> MIKNILGLALGTNSIGWALVKQDFENKQGEILGMGSRIIPMSQDILGDFGKGNSVSQTAERTKYRSVRRLRERFLLRRERLHRVLYILNFLPEHYASQIDFEKRLGKFKVETEPKLVWKNTDGQFSFLFQNSFNEMLEDFKAAGQELKIPYDWTIYHLRKKAISQKIEKEELAWILLNFNHKRGYYQLRGEDFEEEKDKTFVRLKVDRIVDSGENVKGKILYDVYFENGWKYDKQVVKTEDWVDRTKEFIVSESILKNGETKRTFKAVDSEKDWIAIKTKTEQEIEHSHKTVGTYIYETLLQNPKQKIKGKLVRTIERKFYKEELRQILEKQKEFHQELQSDDLYNDCIRELYRNNEVHQLTLRKKDFVHLFMEDIIFYQRPLRSQKSSVSNCTLEFRKYKGENGAEHTQYLKAIPKSNPYYQEFRLWQWIFNLNLYTKDNDENVTKVFLNTTQDFENLFEFLNTRKEVDQKALLKHFKLNEKTHRWNFVEDKKYPCNETKTMISSRLDKVENISDDFLTRDIEQKIWHIIYSVNDKVEYEKALKSFARKHHLDESSFFEAFRKFPPFKSEYGSFSEKAIKKLLPLMRLGKYWNYAEIDKYSRERIQKIITGEYDENIKDKVREKSVHLTIENDFQGLQLWLAQYIVYGRHSEASMIGKWNSANDLEVFLKDFKQHSLRNPIVEQVITETLRVVKDIWLKYGNGTKDFFNEIHIELGREMKLPADDRKKLTNQITENENTNLRIKALLAEMMNDHSVENVRPFSPMQQEILKIYEDGVLKSDIEIEDDILKISKTAQPSSSDLKRYKLWLEQKYKSPYTGQIIPLNKLFTPEYEIEAIIPQSRYFDDSFSNKIICESAVNKLKDNYIGLGFIKQFGGTIIELGFGKSVKVFDTEEYEDFVKKHYANNRGKRNKLLMEDIPEKMIERQLNDTRYISKYISGILSNIVRVEDGSDEGVNSKNIVPGNGKITTQLKQDWGLNDVWNDLILPRFERMNQLTNSKDFTAWNENHQKFLPTVPIEFSKGFSKKRIDHRHHALDALVIACATTDHVNLLNNQSAKSDTKRYDLKKKLMKFEKVVYHHTQTGEKIEREIPKQFLKPWEKFTVDAKHNLESIIVSFKQNLRVINKATNYYEKYVEKDGTKNKERVEQAGTNWAIRKPMHKDTVSGKVDLPWVKVPKGKILTATRKSLDSSFDLKSIGSITDTGIQKILKNYLAFKDGNPELAFSPEGIDDLNKNIEKYNDGKPHQPINKVRVFELGSKFQVGQTGNKKGKYVEAAKGTNLFFAVYEDEKGKRSY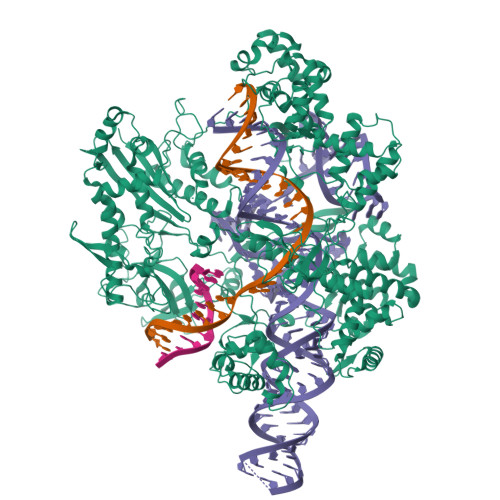ETIPLNEVIERQKQGLTSVPLENEKGSRLLFDLSPNDLVYVPEIDENIDSNFVFSNLNKEKISRIYKVEKTSGTECYFVRQDIAYLIKQYDAKTKIGELESQNKLQVTMTDDRIRITDTCVKINCDRLGNINFITKEKIKQIFNEFR> MGSSHHHHHHSSGLVPRGSYRRKSKQALRDYKKVQIQLENLESSVRDRCKKEFTDLMTEMTDLTSDLLGSGIPFLDYKVYAERIFFPGHRESPLHRDLGVPESRRPTVEQGLGQLSNLLNSKLFLTKFIHTLETQRTFSARDRAYVASLLTVALHGKLEYFTDILRTLLSDLVAQYVAKNPKLMLRRTETVVEKLLTNWMSICLYTFVRDSVGEPLYMLFRGIKHQVDKGPVDSVTGKAKYTLNDNRLLREDVEYRPLTLNALLAVGPGAGEAQGVPVKVLDCDTISQAKEKMLDQLYKGVPLTQRPDPRTLDVEWRSGVAGHLILSDEDVTSEVQGLWRRLNTLQHYKVPDGATVALVPCLTKHVLRENQDYVPGERTPMLEDVDEGGIRPWHLVKPSDEPEPPRPRRGSLRGGERERAKAIPEIYLTRLLSMKGTLQKFV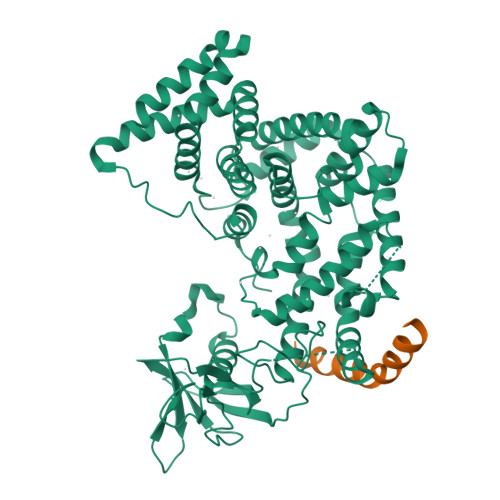DDLFQVILSTSRPVPLAVKYFFDLLDEQAQQHGISDQDTIHIWKTNSLPLRFWINIIKNPQFVFDVQTSDNMDAVLLVIAQTFMDACTLADHKLGRDSPINKLLYARDIPRYKRMVERYYADIRQTVPASDQEMNSVLAELSWNYSGDLGARVALHELYKYINKYYDQIITALEEDGTAQKMQLGYRLQQIAAAVENKVTDL> MSYKQTTYYPSRGNLVRNDSSPYTNTISSETNNSSTSVLSLQGASNVSLGTTGNQLYMGDLDPTWDKNTVRQIWASLGEANINVRMMWNNTLNNGSRSSMGPKNNQGYCFVDFPSSTHAANALLKNGMLIPNFPNKKLKLNWATSSYSNSNNSLNNVKSGNNCSIFVGDLAPNVTESQLFELFINRYASTSHAKIVHDQVTGMSKGYGFVKFTNSDEQQLALSEMQGVFLNGRAIKVGPTSGQQQHVSGNNDYNRSSSSLNNENVDSRFLSKGQSFLSNGNNNMGFKRNHMSQFIY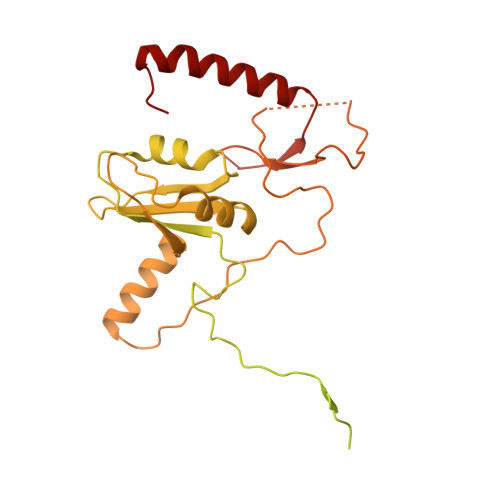PVQQQPSLNHFTDPNNTTVFIGGLSSLVTEDELRAYFQPFGTIVYVKIPVGKCCGFVQYVDRLSAEAAIAGMQGFPIANSRVRLSWGRSAKQTALLQQAMLSNSLQVQQQQPGLQQPNYGYIPSSTCEAPVLPDNNVSSTMLPGCQILNYSNPYANANGLGSNNFSFYSNNNATNTQATSLLADTSSMDLSGTGGQQVIMQGSEAVVNSTNAMLNRLEQGSNGFMFA> MAVYTDITEDELRNFLTQYDVGSLTSYKGIAEGVENSNFLLHTTKDPLILTLYEKRVEKNDLPFFLGLMQHLAAKGLSCPLPLPRKDGELLGELSGRPAALISFLEGMWLRKPEAKHCREVGKALAAMHLASEGFEIKRPNALSVDGWKVLWDKSEERADEVEKGLREEIRPEIDYLAAHWPKDLPAGVIHADLFQDNVFFLGDEL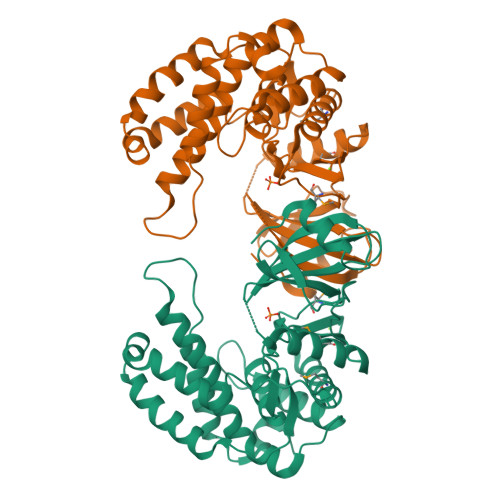SGLIDFYFACNDLLAYDVSICLNAWCFEKDGAYNVTKGKALLEGYQSVRPLSEAELEALPLLSRGSALRFFLTRLYDWLTTPAGALVVKKDPLEYLRKLRFHRTIANVAEYGLAGE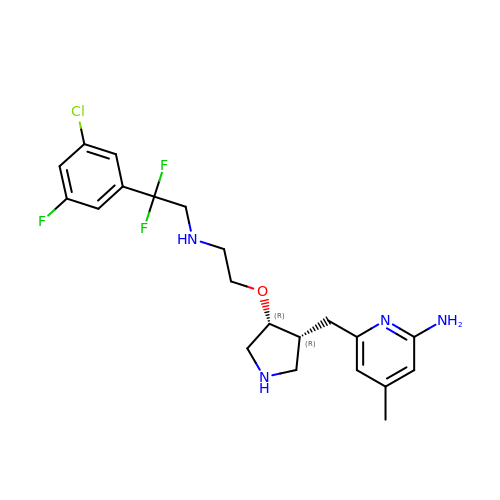6-{[(3R,4R)-4-(2-{[2-(3-chloro-5-fluorophenyl)-2,2-difluoroethyl]amino}ethoxy)pyrrolidin-3-yl]methyl}-4-methylpyridin-2-amine | C21 H26 Cl F3 N4 O | WCMZHGFWPJYQKM-KUHUBIRLSA-N> IPDLIDLD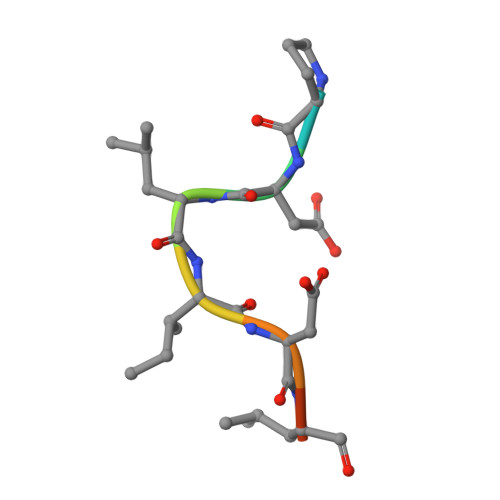D(4E)-4-hydrazinylidene-1,4-dihydroquinoline | C9 H9 N3 | 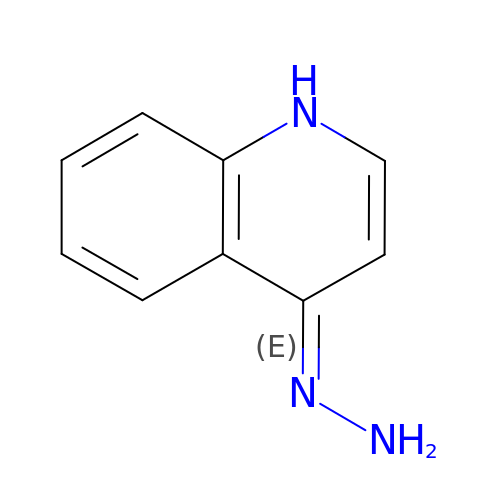MYGFXCLXHGITIQ-UHFFFAOYSA-N>[2x]LPTSNPAQELEARQLERTTRDDLINGNSASCADVIFIYARGSTETGNLGTLGPSIASNLESAFGKDGVWIQGVGGAYRATLGDNALPRGTSSAAIREMLGLFQQANTKCP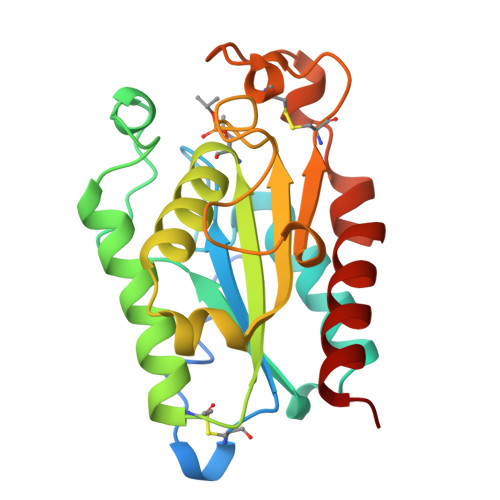DATLIAGGYSQGAALAAASIEDLDSAIRDKIAGTVLFGYTKNLQNRGRIPNYPADRTKVFCNTGDLVCTGSLIVAAPHLAYGPDARGPAPEFLIEKVRAVRGSA> MTKQRDNRVMLITYADSLGADLKELKTALDTWYDKAVGGVHILPFFPSGADRGFSPKTYEMVDPAFGSFADVEAIGKDRWLMFDFMVNHISAQSEYYRDFLEKKEESDWKDFFIRYSKFWPGGAPTQEQVDAIYKRKPRAPYIEAHFADGTEDKVWCTFSEDQIDLDVSSPKVLEFIDRTLDDMADHSASVIRLDAFAYAVKKPGGSCFFEAPEIWQLLDRIESRMQARGVEILPEIHEHYTIPLSLADRGYWIYDFALPVLTLHALYTGNGEYLARWLKMCPKHQYTTLDTHDGLGVVDVRDLLPQEETDRVLDLLYEKGANLNRKYSSEAYGNLDIYQVNTTYYSALGNDDARYLMARAIQFFAPGIPQVYYVGLLAGENDLELLERTRNGRDINRHG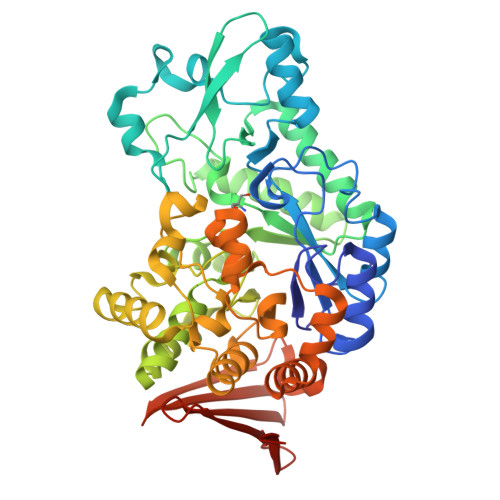YSLEEIEENQKRPVVQDLKWLMELRNSHPAFDLEGDLDVASEDGHLRMLRRSGDEALELDCDLVSGRFTIEDKKRGNRLWPYRLEHHHHHH>[2x]MTHSPSFLQHALSSSDTRAEWPLPGGLAARWLAPGCVELNGDARGADSVLLSCGVHGNETAPIEVVDGMLTDIAAGQLALNCRLLVMFANLDAIRQGVRYGNYDMNRLFNGAHARHPELPESVRAAELETLAAEFFAGARARKLHYDLHTAIRGSVFEKFAIY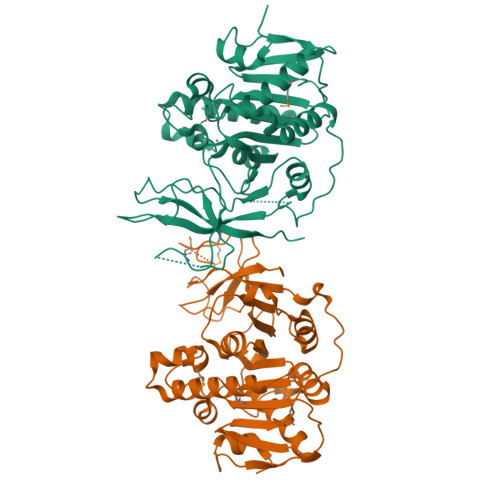PFLHDGRTHKREQLAWLQRCGIEAVLLHTQPANTFSYFTSQYCEADAFTLELGKARPFGQNDLSRFSGIDGALRGLLSNPQANVPDLDEDKLPLFRAKYDLVKHSEAFKLNLADSVENFTLLPDGMLIAEDGAVRYQATGGEERILFPNPAVKPGLRAGIVVEPARLPSRLEHHHHHH AtBFN2 (also called ENDO2) is a 34.5 kDa glycoprotein (the predicted mass for protein component alone is 30.5 kDa), encoded by the Arabidopsis thaliana At1g68290 gene. AtBFN2 follows the standard glycosylation pattern of plant S1/P1 endonucleases, with three glycosylation sites (Asn91, Asn110, and Asn184). While the P1 nuclease has a higher specificity for RNA over ssDNA, in a previous study we showed that the opposite is true for AtBFN2. Structurally, Zn2+-dependent endonucleases present a unique fold, and are classified into the P1/S1 nuclease family (pfam ID PF02265), itself part of the Phospholipase C (PLC)/P1 nuclease superfamily (pfam ID CL0368).

We improved the resolution of our earlier sulfate co-crystal from 1.76 Å to 1.22 Å, thus yielding more insight into the glycan structure. The glycan bound to Asn91 is especially well defined and we can discern both N-acetylglucosamines (GlcNAc), and a further six mannose moieties (Man). Further, the methyl group of GlcNAc1 is located within a small aliphatic pocket formed by Leu57, and Ala88. GlcNAc2, on the other hand, interacts via π-ring stacking with Trp53. While we were able to refine only one additional mannose moiety on the glycan bound to Asn184, we obtained a much more detailed structure for the one attached to Asn110. Interestingly, GlcNAc1 at Asn110 interacts specifically with a single sulfate molecule, which itself interacts with Arg46 and Arg50, and with the aromatic nitrogen of Trp43. The sulfate binding pocket seems well prepared to bind ligands which are both negatively charged and contain de-localized π-orbitals. It is tempting to think that this might be a possible accessory binding site for ssDNA. Pocket two is occupied in the sulfate co-crystal structure by sulfate, suggesting that it should be possible for the ssDNA backbone to be bound in a similar fashion. In the SO4 co-crystal structure, however, only Wat3 remains.

> WGKEGHEIICKIAQTRLDETAAKAVKELLPESAEGDLSSLCLWADRVKFRYHWSSPLHYINTPDACSYQYNRDCKDESGEKGRCVAGAIYNYTTQLLSYKTAASSQSQYNLTEALLFVSHFMGDIHQPLHVSYASDKGGNTIEVHWYTRKANLHHIWDSNIIETAEADLYNSALEGMVDALKKNITTEWADQVKRWETCTKKTACPDIYASEGIQAACDWAYKGVTEGDTLEDEYFYSRLPIVYQRLAQGGVRLAATLNRIFGHHHHHH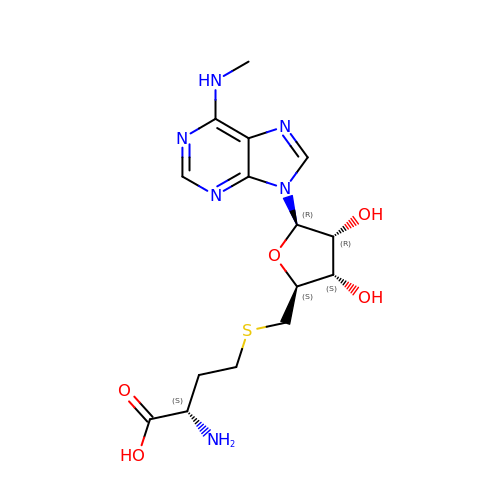(2S)-2-azanyl-4-[[(2S,3S,4R,5R)-5-[6-(methylamino)purin-9-yl]-3,4-bis(oxidanyl)oxolan-2-yl]methylsulfanyl]butanoic acid | C15 H22 N6 O5 S | GEJILRRXJVSBCM-TWBCTODHSA-N2-[2-[2-[2-[2-(2-hydroxyethyloxy)ethoxy]ethoxy]ethoxy]ethoxy]ethanoic acid | C12 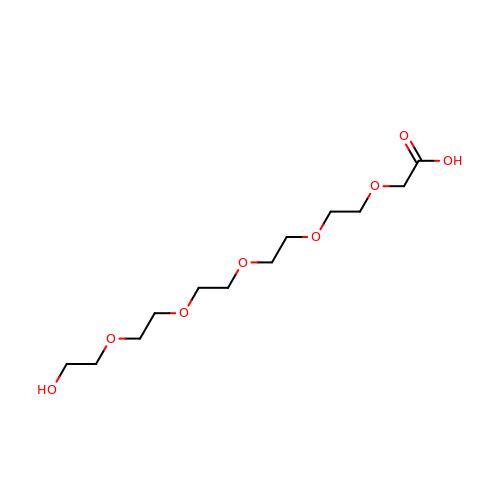H24 O8 | SXGGZTBEWZFLBZ-UHFFFAOYSA-N> HHHHHHTDPQGDAAQKTDTSHHDQDHPTFNKITPNLAEFAFSLYRQLAHQSNSTNIFFSPVSIATAFAMLSLGTKADTHDEILEGLNFNLTEIPEAQIHEGFQELLRTLNQPDSQLQLTTGNGLFLSEGLKLVDKFLEDVKKLYHSEAFTVNFGDTEEAKKQINDYVEKGTQGKIVDLVKELDRDTVFALVNYIFFKCKWERPFEVKDTEEEDFHVDQVTTVKVPMMKRLGMFNIQHCKKLSSWVLLMKYLGNATAIFFLPDEGKLQHLENELTHDIITKFLENEDRRSASLHLPKLSITGTYDLKSVLGQLGITKVFSNGADLSGVTEEAPLKLSKAVHKAVLTIDEKGTEAAGAMFLEAIPMSIPPEVKFNKPFVFLMIEQNTKSPLFMGKVVNPTQK

Mutants of alpha‐1‐antitrypsin cause the protein to self‐associate and form ordered aggregates (‘polymers’) that are retained within hepatocytes, resulting in a predisposition to the development of liver disease. The associated reduction in secretion, and for some mutants, impairment of function, leads to a failure to protect lung tissue against proteases released during the inflammatory response and an increased risk of emphysema. We report here a novel deficiency mutation (Gly192Cys), that we name the Sydney variant, identified in a patient in heterozygosity with the Z allele (Glu342Lys).

X‐ray crystallography provided two crystal structures of the Gly192Cys variant, revealing perturbation within the ‘breach’ region with Cys192 in two different orientations: in one structure it faces towards the hydrophobic core while in the second it is solvent‐exposed. This orientational heterogeneity was confirmed by PEGylation. Cellular analysis revealed that the novel variant was mostly retained as insoluble polymers within the endoplasmic reticulum. The variant showed a 40% reduction in inhibitory activity and a reduced stability as assessed by thermal unfolding experiments. Polymerisation involves adoption of an aggregation‐prone intermediate and paradoxically the energy barrier for transition to this state was increased by 16% for the Gly192Cys variant with respect to the wild‐type protein. However, with activation to the intermediate state, polymerisation occurred at a 3.8‐fold faster rate overall.> GGGRMDAATTRVGLTDLTFRLLRESFADAVSWVAKNLPARPAVPVLSGVLLTGSDNGLTISGFDYEVSAEAQVGAEIVSPGSVLVSGRLLSDITRALPNKPVDVHVEGNRVALTCGNARFSLPTMPVEDYPTLPTLPEETGLLPAELFAEAISQVAIAAGRDDTLPMLTGIRVEILGETVVLAATDRFRLAVRELKWSASSPDIEAAVLVPAKTLAEAAKAGIGGSDVRLSLGTGPGVGKDGLLGISGNGKRSTTRLLDAEFPKFRQLLPTEHTAVATMDVAELIEAIKLVALVADRGAQVRMEFADGSVRLSAGADDVGRAEEDLVVDYAGEPLTIAFNPTYLTDGLSSLRSERVSFGFTTAGKPALLRPVSGDDRPVAGLNGNGPFPA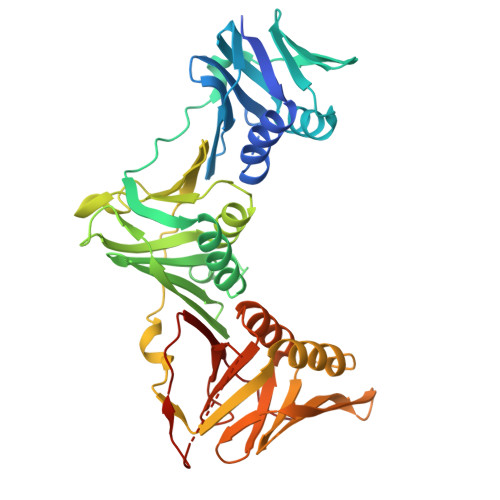VSTDYVYLLMPVRLPG>[2x]MAEIPKEHLRAQTNVILLNVLKQGDNYVYGIIK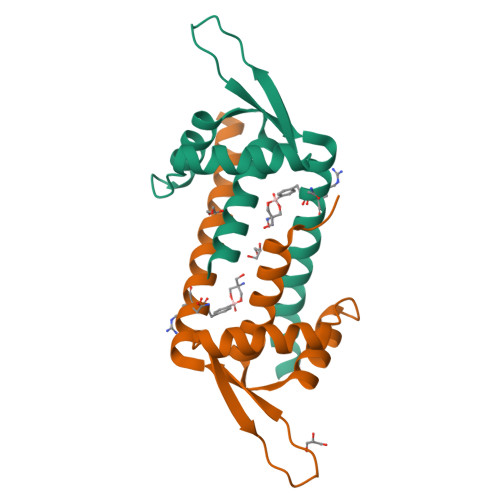QVKEASNGEMELNEATLYTIFKRLEKDGIISSYWGDESQGGRRKYYRLTEIGHENXRLLEESWSRVDKIIENLEANKKSEAIKSRGGSGGWSHPQFEK> MYEGNNMRSMMGT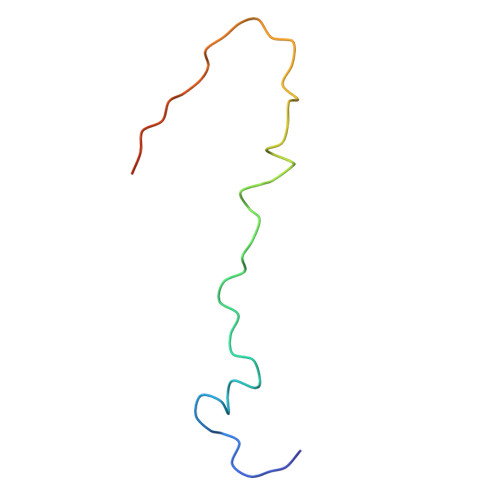SYEDSRLNKRTELNENMSIDTNKSEDSYGVQIHSLSKQSFTGDVEEE> SDKIIHLTDDSFDTDLVKADGAILVDFWAEWCGPCKMIAPILDEIADEYQGKLTVAKLNIDQNPGTAPK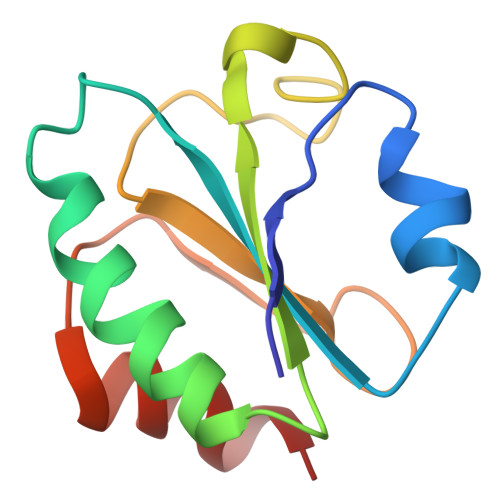YIERGIPTLLLFKNGEVAATKVGALSKGQLKEFLDANLA> MSDNDELQQIAHLRREYTKGGLRRRDLPADPLTLFERWLSQACEAKLADPTAMVVATVDEHGQPYQRIVLLIHYDEKGMVFYTNLGSRKAHQIENNPRVSLLFPWHTLERQVMVIGKAERLSTLEVMKFFHSLPRDS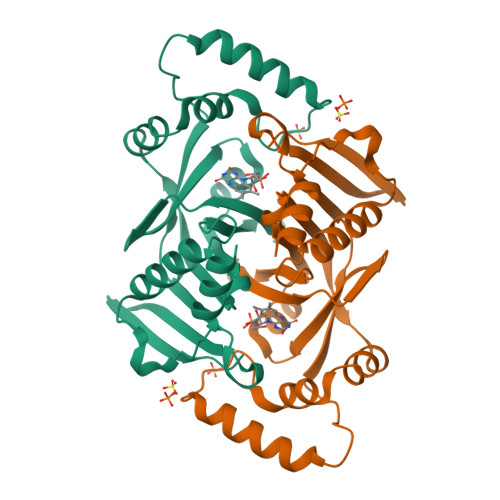QIGAWVSKQSSRISARGILESKFLELKQKFQQGEVPLPSFWGGFRVSLEQIEFWQGGEHRLADRFLYQRENDAWKIDRLAP> MKEVARVRNLNRIIMGKYEIEPWYFSPYPIELTD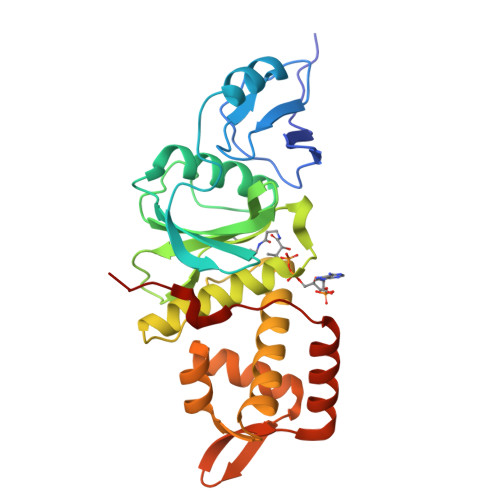EDFIYIDDFTLQYFGSKKQYERYRKKCTLRHPPGNEIYRDDYVSFFEIDGRKQRTWCRNLCLLSKLFLDHKTLYYDVDPFLFYCMTRRDELGHHLVGYFSKEKESADGYNVACILTLPQYQRMGYGKLLIEFSYELSKKENKVGSPEKPLSDLGLLSYRAYWSDTLITLLVEHQKEITIDEISSMTSMTTTDILHTAKTLNILRYYKGQHIIFLNEDILDRYNRLKAKKRRTIDPNRLIWKPPV>[2x]MTNIEPVIIETRLELIGRYLDHLKKFENISLDDYLS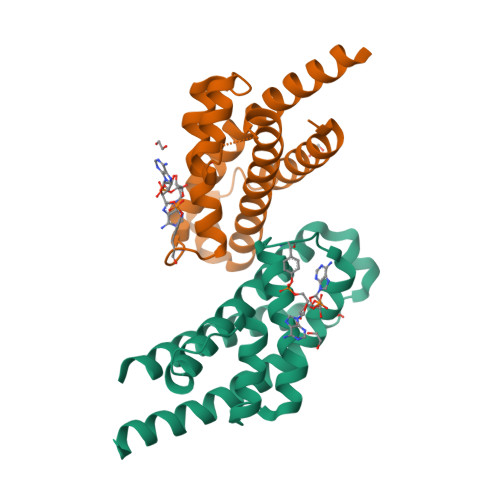SFEQQLITERLLQLITQAAIDINDHILSKLKSGKSYTNFEAFIELGKYQILTPELAKQIAPSSGLANRLVHEYDDIDPNQVFMAISFALQQYPLYVRQINSYLITLEEENDLESGHHHHHH>[2x]PKFFYIKSELNGKVLDIGGQNPAPGSKIITWDQKKGPTAVNQLWYTDQQGVIRSKLNDFAIDASHEQIETQPFDPNNP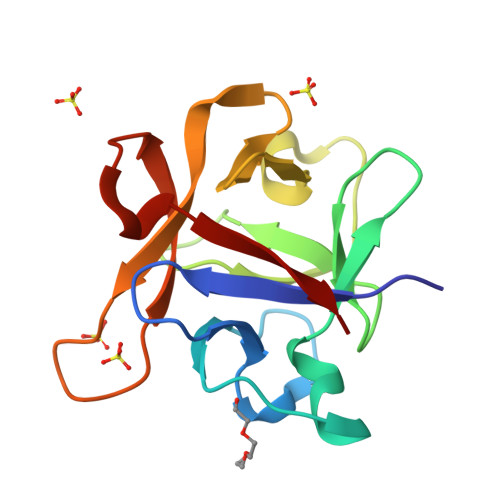KRAWIVSGNTIAQLSDRDNVLGVIKSDKGASAHICAWKQHGGPNQKFIIESE>MSEITLGRYLFERLKQVEVQTIFGLPGDFNLSLLDNIYEVPG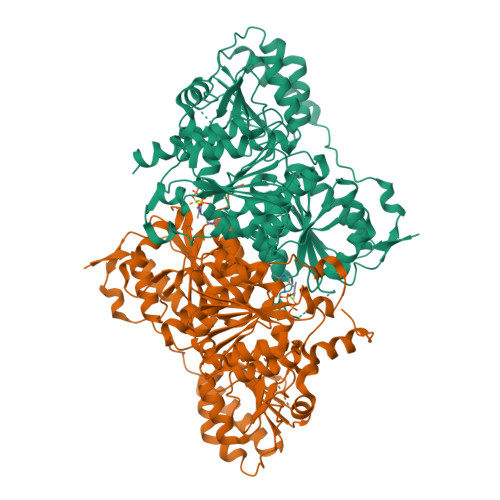MRWAGNANELNAAYAADGYARLKGMSCIITTFGVGELSALNGIAGSYAEHVGVLHVVGVPSVSSQAKQLLLHHTLGNGDFTVFHRMSSNISETTAMITDINTAPAEIDRCIRTTYVSQRPVYLGLPANLVDLTVPASLLDTPIDLSLKPNDPEAEEEVIENVLQLIKEAKNPVILADACCSRHDAKAETKKLIDLTQFPAFVTPMGKGSIDEKHPRFGGVYVGTLSSPAVKEAVESADLVLSVGALLSDFNTGSFSYSYKTKNIVEFHSDYTKIRSATFPGVQMKFALQKLLTKVADAAKGYKPVPVPSEPEHNEAVADSTPLKQEWVWTQVGEFLREGDVVITETGTSAFGINQTHFPNNTYGISQVLWGSIGFTTGATLGAAFAAEEIDPKKRVILFIGDGSLQLTVQEISTMIRWGLKPYLFVLNNDGYTIERLIHGETAQYNCIQNWQHLELLPTFGAKDYEAVRVSTTGEWNKLTTDEKFQDNTRIRLIEVMLPTMDAPSNLVKQAQLTAATNAKN[4x]4-butyl-7,8-bis(oxidanyl)chromen-2-one | C13 H14 O4 | 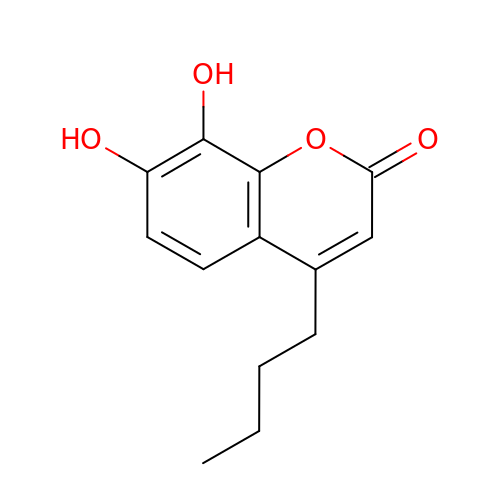GDGBIWNBPUQGGZ-UHFFFAOYSA-N>[4x]HHHHHHNKDLKGLYAALLVPFDENGQVNEQGLKQIAQNAIETEELDGLYVNGSSGENFLLNTEQKKQVFKVAKEAVGDKVKLIAQVGSLDLNEAIELGKYATELGYDALSAVTPFYYPFTFEEIRDYYFDIIEATQNNMIIYAIPDLTGVNISIEQFSELFNHEKIVGVCYTAPNFFLLERIRKAFPDKLILSGFDEMLVQATISGVDGAIGSTYNVNGRRARKIFDLARQGQIQEAYQLQHDSNDIIETVLSMGIYPTLKEILRHRGIDAGLPKRPFKPFNEAHRQTLDQLIAKYDL

NAL catalyses the reversible aldol condensation of N-acetylmannosamine with pyruvate to yield the sialic acid, N-acetylneuraminic acid (Neu5Ac). NAL is a class I aldolase, functioning through the formation of an enzyme–pyruvate Schiff base formed with Lys165 which carries out a nucleophilic attack on the aldehyde carbon of the open-chain form of the N-acetylmannosamine. Here, using the NAL from Staphylococcus aureus, we demonstrate quantitative conversion of a cysteine residue, site-specifically into the nonproteogenic amino acid γ-thialysine, chosen as a mimic of the natural catalytic lysine residue at position 165, using the double alkylation-elimination method and that high yields of an active, modified NAL can be purified. We then characterise the resulting enzyme activity, analyse the pH-dependency of catalysis and use X-ray crystallography to investigate the structural basis of the changes brought about by modifying the enzyme.

A mutant nanA gene encoding the K165C S. aureus NAL was created using site-directed mutagenesis and DNA sequencing confirmed the presence of the mutation. The structure of the K165C variant showed no significant changes in the overall structure of the protein compared with the wild-type enzyme (RMSD over all Cα atoms=0.34 Å). However, the observed electron density for residue 165 did not extend far enough for a lysine residue and was better fitted by a cysteine residue as expected. Interestingly, the K165C structure more closely resembled the enzyme–pyruvate complexes than the apo structures since the loop region (138–146), not generally resolved in apo structures, could be clearly seen in the structure of the K165C variant and the side chain of Tyr137 was also positioned more similarly to that in the pyruvate complexes. Calculation of side-chain solvent accessibility for the K165C variant showed that the cysteine is inaccessible explaining the need to unfold the protein prior to chemical modification. Despite soaking K165C crystals with up to 100 mm pyruvate, we were never able to observe electron density for substrate in the enzyme active site. Experiments demonstrated that the cysteine side chain in the native protein was inaccessible to the reagent 2,5-dibromo-1,6-hexadiamide used to generate the dehydroalanine residue. Nevertheless, replacement of the natural lysine side chain with a thialysine residue is still consistent with activity and the rate of the reaction is enhanced 360-fold when compared with the inactive K165C variant.>MGALESLRGNADLAYILSMEPCGHCLIINNVNFCRESGLRTRTGSNIDCEKLRRRFSSLHFMVEVKGDLTAKKMVLALLELARQDHGALDCCVVVILSHGCQASHLQFPGAVYGTDGCPVSVEKIVNIFNGTSCPSLGGKPKLFFIQACGGEQKDHGFEVASTSPEDESPGSNPEPDATPFQEGLRTFDQLDAISSLPTPSDIFVSYSTFPGFVSWRDPKSGSWYVETLDDIFEQWAHSE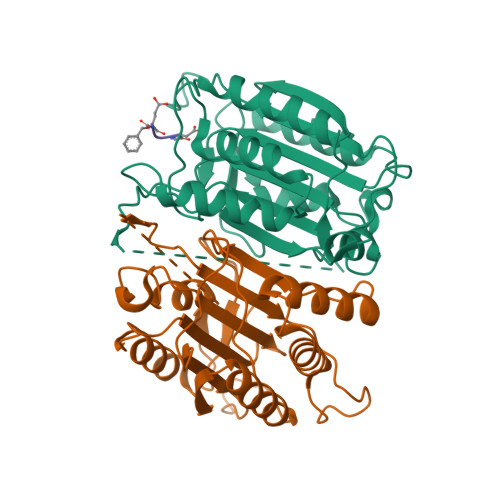DLQSLLLRVANAVSVKGIYKQMPGCFNFLRKKLFFKTSHHHHHH[4x]>MGHHHHHHHHSSGHIEGRHMAHLLIVNVASHGLILPTLTVVTELVRRGHRVSYVTAGGFAEPVRAAGATVVPYQSEIIDADAAEVFGSDDLGVRPHLMYLRENVSVLRATAEALDGDVPDLVLYDDFPFIAGQLLAARWRRPAVRLSAAFASNEHYSFSQDMVTLAGTIDPLDLPVFRDTLRDLLAEHGLSRSVVDCWNHVEQLNLVFVPKAFQIAGDTFDDRFVFVGPCFDDRRFLGEWTRPADDLPVVLVSLGTTFNDRPGFFRDC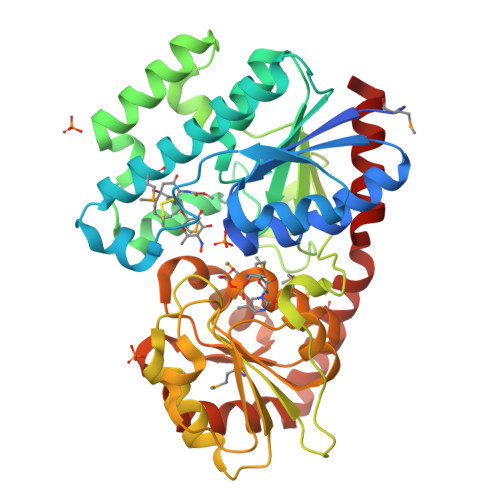ARAFDGQPWHVVMTLGGQVDPAALGDLPPNVEAHRWVPHVKVLEQATVCVTHGGMGTLMEALYWGRPLVVVPQSFDVQPMARRVDQLGLGAVLPGEKADGDTLLAAVGAVAADPALLARVEAMRGHVRRAGGAARAADAVEAYLARA[2x]>MINKDTQLCMSLSGRPSNFGTTFHNYLYDKLGLNFIYKAFTTQDIEHAIKGVRALGIRGCAVSMPFKETCMPFLDEIHPSAQAI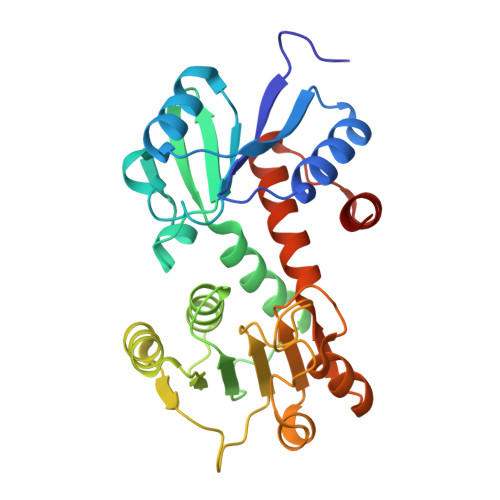ESVNTIVNDNGFLRAYNTDYIAIVKLIEKYHLNKNAKVIVHGSGGMAKAVVAAFKNSGFEKLKIYARNVKTGQYLAALYGYAYINSLENQQADILVNVTSIGMKGGKEEMDLAFPKAFIDNASVAFDVVAMPVETPFIRYAQARGKQTISGAAVIVLQAVEQFELYTHQRPSDELIAEAAAFARTKF[4x]Immunoglobulin (Ig) A functions as monomeric IgA in the serum and Secretory (S) IgA in mucosal secretions. Host IgA Fc receptors (FcαRs), including human FcαR1/CD89, mediate IgA effector functions; however, human pathogen Streptococcus pyogenes has evolved surface-protein virulence factors, including M4, that also engage the CD89-binding site on IgA. SIgA is polymeric and is typically composed of two mIgA that assemble with one joining-chain (JC) to form dimeric (d) IgA, which is bound by the polymeric Ig-receptor (pIgR) ectodomain, called secretory component (SC). Here we report cryo-EM structures of M4-SIgA and CD89-SIgA complexes, which unexpectedly reveal different SIgA-binding stoichiometry for M4 and CD89.

In order to better understand how bacterial virulence factors such as M4 engage SIgA, we designed an M4 expression construct encoding the ectodomain (residues 1–314) and combined the resulting protein with purified, recombinant human SIgA1 to create an SIgA-M4 complex. Using this complex, we determined the SIgA-M4 cryo-EM structure to an average resolution of 3.1 Å (FSC = 0.143). The final structure included a single M4 dimer bound to one SIgA; M4 residues 45–73, which include the entire known IgA-binding domain, were built whereas the positions of residues more distal from the binding site were poorly resolved or disordered, likely due to the inherent flexibility of the M4 dimer’s extended, coiled-coil structure. A subset of residues between P46-K68 in both helices contact SIgA, with one (helix-a) forming the majority of contacts with the IgA heavy chain and the other (helix-b) using equivalent residues to contact solvent and a smaller interface with IgA. The M4 interface includes 11 residues on the Cα3 domain of both heavy chain-A (HC-A) and heavy chain-B (HC-B), with a total buried surface area of 1000 Å2. Participating IgA residues are predominantly located along one β-strand in HC-A (F443, T444, Q445, T447), forming hydrogen bonds with M4 helix-a residues R49 and E54. HC-A E389 and R346 also reach out to interact with M4 helix-a residues Q47 and D57, respectively, and HC-A D449 forms a salt bridge with R59 on helix-b of M4. The M4 interface with IgA HC-B includes only residues S356, E357 and A360, which form hydrogen bonds with Q66 of helix-b and R61, K68 of helix-a, respectively. In the case of M4, the inclusion of S356, E357, A360 and R346 in the M4 binding interface, together with its extended coiled-coiled topology, enforce the surprising 1M4:1SIgA stoichiometry because the steric accessibility of these four residues and neighboring residues differs between FcAB and FcCD. In FcCD, S356, E357, A360 and R346 remain solvent accessible, but JC loop residues 24–32 bind the adjacent region, blocking the path occupied by M4 (helix-b residues 69–72) and therefore occluding binding.

>[4x]ASPTSPKVFPLSLCSTQPDGNVVIACLVQGFFPQEPLSVTWSESGQGVTARNFPPSQDASGDLYTTSSQLTLPATQCLAGKSVTCHVKHYTNPSQDVTVPCPVPSTPPTPSPSTPPTPSPSCCHPRLSLHRPALEDLLLGSEANLTCTLTGLRDASGVTFTWTPSSGKSAVQGPPERDLCGCYSVSSVLPGCAEPWNHGKTFTCTAAYPESKTPLTATLSKSGNTFRPEVHLLPPPSEELALNELVTLTCLARGFSPKDVLVRWLQGSQELPREKYLTWASRQEPSQGTTTFAVTSILRVAAEDWKKGDTFSCMVGHEALPLAFTQKTIDRLAGKPTHVNVSVVMAEVDGTCY;> KSPIFGPEEVNSVEGNSVSITCYYPPTSVNRHTRKYWCRQGARGGCITLISSEGYVSSKYAGRANLTNFPENGTFVVNIAQLSQDDSGRYKCGLGINSRGLSFDVSLEVSQGPGLLNDTKVYTVDLGRTVTINCPFKTENAQKRKSLYKQIGLYPVLVIDSSGYVNPNYTGRIRLDIQGTGQLLFSVVINQLRLSDAGQYLCQAGDDSNSNKKNADLQVLKPEPELVYEDLRGSVTFHCALGPEVANVAKFLCRQSSGENCDVVVNTLGKRAPAFEGRILLNPQDKDGSFSVVITGLRKEDAGRYLCGAHSDGQLQEGSPIQAWQLFVNEESTIPRSPTVVKGVAGGSVAVLCPYNRKESKSIKYWCLWEGAQNGRCPLLVDSEGWVKAQYEGRLSLLEEPGNGTFTVILNQLTSRDAGFYWCLTNGDTLWRTTVEIKIIEGEPNLKVPGNVTAVLGETLKVPCHFPCKFSSYEKYWCKWNNTGCQALPSQDEGPSKAFVNCDENSRLVSLTLNLVTRADEGWYWCGVKQGHFYGETAAVYVAVEERHHHHHH;> QEDERIVLVDNKCKCARITSRIIRSSEDPNEDIVERNIRIIVPLNNRENISDPTSPLRTRFVYHLSDLCKKCDPTEVELDNQIVTATQSNICDEDSATETCYTYDRNKCYTAVVPLVYGGETKMVETALTPDACYPD;>AEIKKPQADSAWNWPKEYNALLKENEELKVEREKYLSYADDKEKDPQYRALMGENQDLRKREGQYQDKIEELEKERKEKQERQEQLERQYQIEADKHYQEQQKKHQQEQQQLEAEKQKLAKDKQISDASRQGLSRDLEASRAAKKELEAEHQKLKEEKQISDASRQGLSRDLEASREAKKKVEADLAALTAEHQKLKEDKQISDASRQGLSRDLEASREAKKKVEADLAEANSKLQALEKLNKELEEGKKLSEKEKAELQARLEAEAKALKEQLAKQAEELAKLKGNQTPNAKVAPQANRSRSAMTQQKRTLPSTHHHHHH[2x]> SRLDKSKVINSALELLNEVGIEGLTTRKLAQKLGVEQPTLYWHVKNKRALLDALAVEILARHHDYSLPAAGESWQSFLRNNAMSFRRALL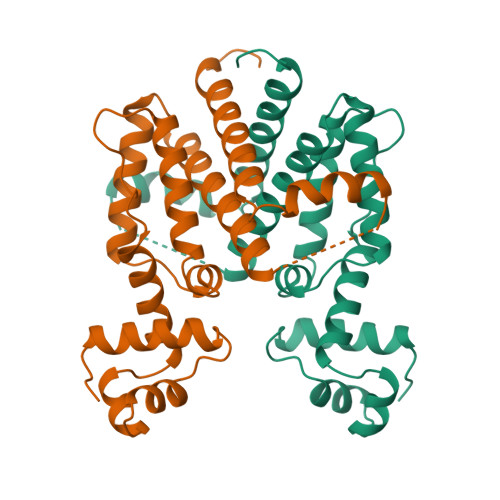RYRDGAKVHLGTRPDEKQYDTVETQLRFMTENGFSLRDGLYAISAVSHFTLGAVLEQQEHTAALTDRPAAPDENLPPLLREALQIMDSDDGEQAFLHGLESLIRGFEVQLTALLQIVGGDKLIIPFC>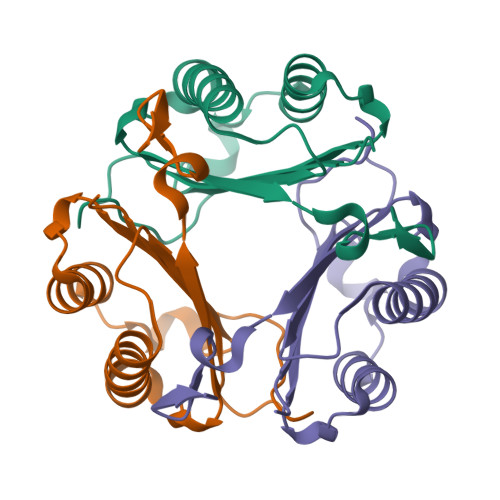[8x]PAAAMFIVNTNVPRASVPDGFLSELTQQLAQATGKPPQYIAVHVVPDQLMAFGGSSEPCALCSLHSIGKIGGAQNRSYSKLLCGLLAERLRISPDRVYINYYDMNAANVGWNNSTFA>[4x]MKHHHHHHSAGLEVLFQGPDSMDKQVSKLQRKNKAKQLRAQRILDSIENRKLFEGKNGAAKIITIVPLVNDLDPLDILYKLLKCADDEGIMVQEVDSKRIFNVHIKKFKSNLKIIIPDMTNFLNILDCAKVADFVVFGLSGVQEVDEEFGEQIIRALELQGIASYIGVISNLSAVHEKEKFQLDVKQSLESYFKHFFPSEERVYNLEKNSDALNVLRTLCQRLPRSINWRDNRGYVVADFVDFVETSPDSGDLVIEGTVRGIGFNANRLVHIPDFGDFQLNKIEKISESSQKRKIIKEKATDSLSLELDLQTVFE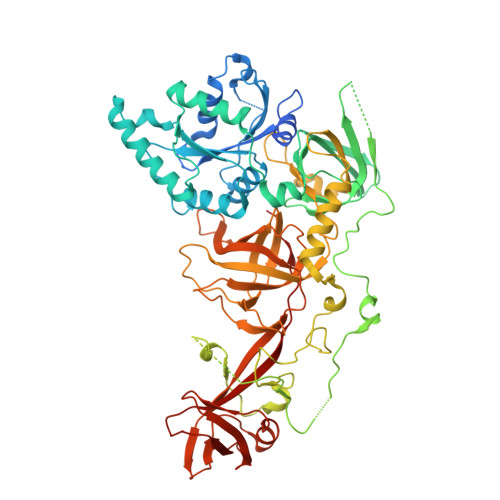SNMNRDTLDEYAPEGTEDWSDYDEDFEYDGLTTARYDDHGFLPGREQTSKKAAVPKGTSDYQAKWYLDDVIPSSGSSKEDREFPDEIELEPSESAIERLKRYRGLKNLYNCDWQVDEKDPSSPAEWKRLLRIGNYKNTKNRIIKETKNEAQAIAGDRIRMFIRFPKFLLEKIQDPKQLLFAVYGLLLHEHKNAVVNFSLQRWEQYDKPVPSQEPIVVQYGVRRYTIQPLFSQGSNSPNNVHKYERFLHPDTVSVATCIAPVDFTQSPAIFFKPSPTDAKNIELIGHGTFLNADHSRILAKRAILTGHPFRFHKTVVTVRYMFFRPEDVEWFKSIPLFTKSGRSGFIKESLGTHGYFKATFDGKLSAQDVVAMSLYKRMWPMPSLPWNGM> MAKVEQVLSLEPQHELKFRGPFTDVVTTNLKLGNPTDRNVCFKVKTTVPRRYCVRPNSGVIDAGASLNVSVMLQ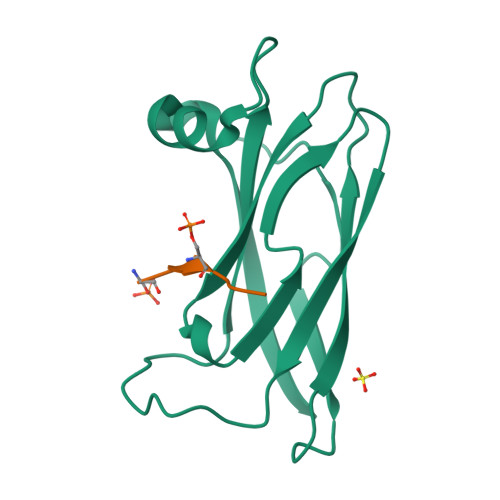PFDYDPNEKSKHKFMVQSMFAPPDTSDMEAVWKEAKPEDLMDSKLRCVFEL;> SEDSFFSATE> FQFVTPVGTQNGLKATCAKISPDGQFLAITQGLNILIYDINRRTVSQTLVTSHARPFSELCWSPDGQCIATASDDFSVEIIHLSYGLLHTFIGHTAPVISLTFNRKGNLLFTSSMDESIKIWDTLNGSLMKTISAHSEAVVSVDVPMNDSSILSSGSYDGLIRIFDAETGHCLKTLTYDKDWKRENGVVPISQVKFSENARYLLVKSLDGVVKIWDCIGGCVVRTFQVQPLEKGVLHHSCGMDFLNPEDGSTPLVISGYENGDIYCWNSDTKSLLQLLDGSLYHHSSPVMSIHCFGNIMCSLALNGDCCLWRWV;> NILLQDPFAVLKEHPEKLTHTIENPLRTECLQFSPCGDYLALGCANGALVIYDMDTFRPICVPGNMLGAHVRPITSIAWSPDGRLLLTSSRDWSIKLWDLSKPSKPLKEIRFDSPIWGCQWLDAKRRLCVATIFEESDAYVIDFSNDPVASLLSKSDEKQLSSTPDHGYVLVCTVHTKHPNIIIVGTSKGWLDFYKFHSLYQTECIHSLKITSSNIKHLIVSQNGERLAINCSDRTIRQYEISIDDENSAVELTLEHKYQDVINKLQWNCILFSNNTAEYLVASTHGSSAHELYIWETTSGTLVRVLEGAEEELIDINWDFYSMSIVSNGFESGNVYVWSVVIPPKWSALAPDFEEVEENVDYLEKEDEFDEVDEAEQQQGLEQEEEIAIDLRTREQYDVRGNNLLVERFTI;> KIWQSRRKTLEEEKASDWQIELNGTLFDSELQPGSSFKAEGFRKVTDKLKINYLPHRRRVHQPLNTVNIHNERNEYTPELCQREESSNKEPSDSVPQEVSSSRDNRASNRRFQQDIEAQKAAIGTESELLSLNQLNKRKKPVMFARSAIHNWGLYALDSIAAKEMIIEYVGERIRQPVAEMREKRYLKNGIGSSYLFRVDENTVIDATKKGGIARFINHCCDPNCTAKIIKVGGRRRIVIYALRDIAASEELTYDYKFEREKDDEERLPCLCGAPNCK;> HGREFVNDIWSRLKTDEDRAVVKKMVEQTGHIDKFKKFGQLDFIDNNIVVKTDDEKEIFDQIVVRDMTLKTLEDDLQEVQEISLPLFKKKLELLEVYLGWLDNVYTEMRKLDDDAASHVECGKEDSKGTKRKKKKNSSRSRARKNICGYCSTYERIPCSVEEFVRDFGSNEEATKIHEVCTKWKCNRHLDWVSTNQEQYLQQIDSLESMQERLQHLIQARKKQLNIQYYEEILRRGL;> FDHSGMSVMDRSEGLSISRDGNDLVSVPDQYGWR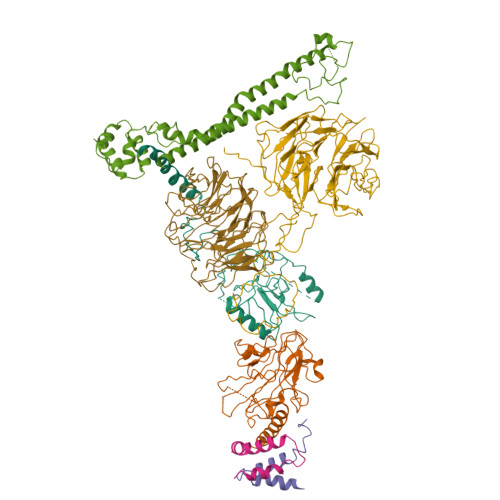TARSDVCIKEGMTYWEVEVIRGGNKKFADGVNNKENADDSVDEVQSGIYEKMHKQVNDTPHLRFGVCRREASLEAPVGFDVYGYGIRDISLESIHEGKLNCVLENGSPLKEGDKIGFLLSLPSIHTQIKQAKEFTKRRIFALNSHMDTMNEPWREDAENGPSRKKLKQETTNKEFQRALLEDIEYNDVVRDQIAIRYKNQLFFEATDYVKTTKPEYYSSDKRERQDYYQLEDSYLAIFQNGKYLGKAFENLKPLLPPFSELQYNEKFYLGYWQHGEARDESNDKNTTSAKKKKQQQKKKKGLILRNKYVNNNKLGYYPTISCFNGGTARIISEEDKLEYLDQIRSAYCVDGNSKVNTLDTLYKEQIAEDIVWDIIDELEQIAL;>TRKYLNTNVTPHLLAGMRLIAVQQPEDPLRVLGEYLIEQSNI[2x]One important example is the biosynthesis of human ABO blood group antigens, which is the most important blood group system in transfusion and transplantation. GTA catalyzes the transfer of GalNAc from UDP-GalNAc to the H antigen acceptor (HAA) (α-l-Fuc-(1→2)-β-d-Gal-O-R, where R is glycolipid or glycoprotein) to form the A antigen, whereas GTB catalyzes the transfer of Gal from UDP-Gal to the HAA to form the B antigen. Among these is the enzyme AAGlyB, a dual-specificity GT, which can bind and utilize either UDP-Gal or UDP-GalNAc with equal efficiency. Each letter corresponds to one critical residue in increasing order such that the AAGlyB chimer would correspond to GTA-L266G/G268A.

Three of the structures belong to space group P21212 containing 2 molecules in the asymmetric unit whereas the fourth one, the AAGlyB-2 complex, belongs to space group C2221 with only one molecule in the asymmetric unit. The single chain in the AAGlyB-2 structure shares the least similarity to the other structures. In the AAGlyB-2 and AAGlyB-2-HAA complexes where the 5-substituent of the donor analogue is a phenyl group, the electron density is well defined throughout most of the only chain in the AAGlyB-2 structure and chain A and B in the AAGlyB-2-HAA structure. Finally, as for the AAGlyB-1 structure, the AAGlyB-2 shows well defined density for the galactose in the tucked under conformation, whereas in the AAGlyB-2-HAA structure the galactose is not visible except for a few blobs extending out from the nucleotide β-phosphate. UDP-Gal derivative 2, which differs from 1 in the nature of the 5-substituent, has a Km value that is approximately 10-fold higher than that of both the parent UDP-Gal and UDP-Gal derivative 1. The kcat of 2 is 1–2% of UDP-Gal and lower than that of 1, by a factor of 4. These results suggest that the 5-phenyl substituent in 2 is less well tolerated at the donor binding site of AAGlyB than the 5-formylthienyl substituent in 1 and disfavors the binding of donor analogue 2 in a catalytically productive orientation.

> MAIGEFMVSLPRMVYPQPKVLTPCRKDVLVVTPWLAPIVWEGTFNIDILNEQFRLQNTTIGLTVFAIKKYVAFLKLFLETAEKHFMVGHRVHYYVFTDQPAAVPRVTLGTGRQLSVLEVRAYKRWQDVSMRRMEMISDFCERRFLSEVDYLVCVDVDMEFRDHVGVEILTPLFGTLHPGFYGSSREAFTYERRPQSQAYIPKDEGDFYYGGAFFGGSVQEVQRLTRACHQAMMVDQANGIEAVWHDESHLNKYLLRHKPTKVLSPEYLWDQQLLGWPAVLRKLRFTAVPKNHQAVRNP> GAMSQDDDYLYCEKCQNFFIDSCPNHG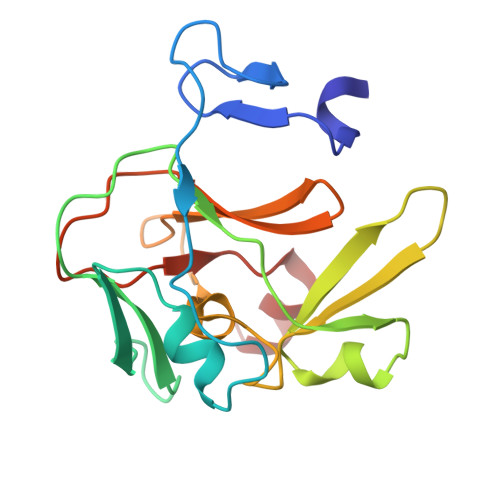PPLFVKDSMVDRGHPNHSVLSLPPGLRISPSGIPEAGLGVWNEASDLPVGLHFGPYEGQITEDEEAANSGYSWLITKGRNCYEYVDGQDESQANWMRYVNCARDDEEQNLVAFQYHRKIFYRTCRVIRPGCELLVWYGDEYGQELGIK> MANNNEIDPLLTLELSGVKTYESQEEAWGARLYEWLNTYQGEVYGDPSWGNVLPQFKHEPTNLSHVQIAVEAMLLQKLTVDLPDIPISGLSVAEGDAFDKLKISIRIRDIT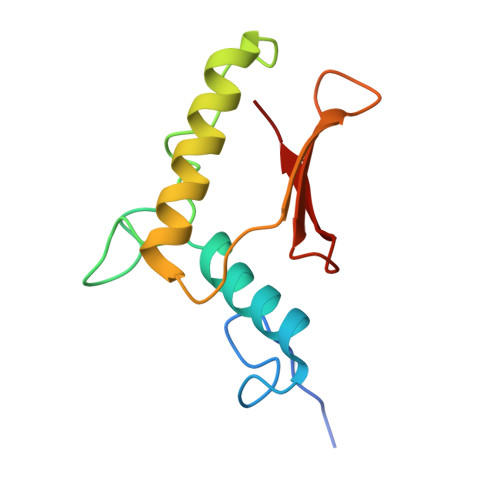ITQDVVL4,4'-sulfanediylbis{N-[(1E)-pyridin-2-ylmethylidene]aniline} | 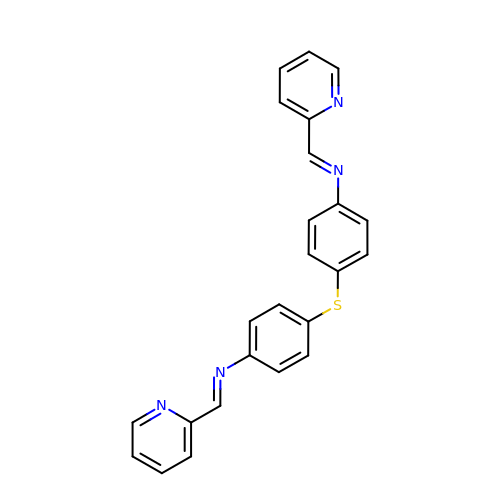C24 H18 N4 S | KHOHHSYBCGDFBZ-XUIWWLCJSA-N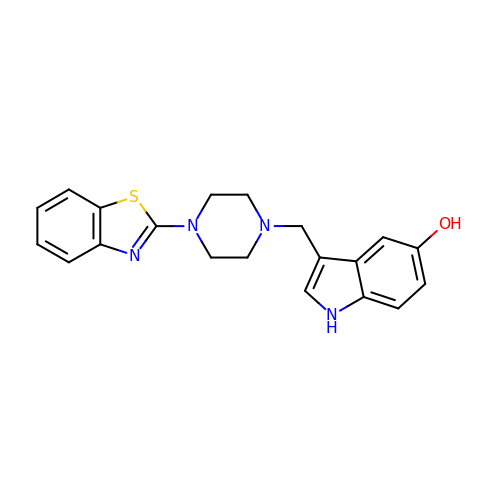3-[[4-(1,3-benzothiazol-2-yl)piperazin-1-yl]methyl]-1~{H}-indol-5-ol | C20 H20 N4 O S | RXEWNCAVTJMLIP-UHFFFAOYSA-N N-[(3M)-3-(5-chloro-1,2,3-thiadiazol-4-yl)phenyl]-5-methyl-3-oxo-2,3-dihydro-1,2-oxazole-4-sulfonamide | C12 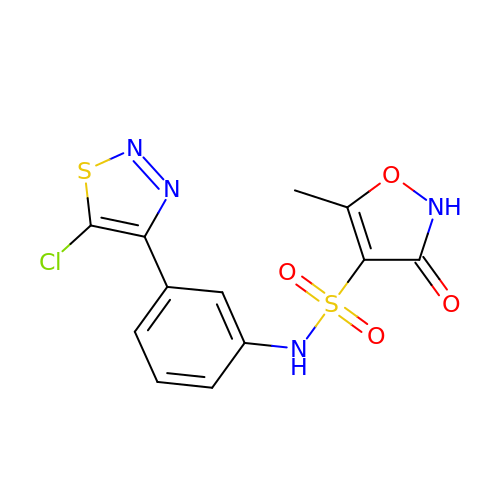H9 Cl N4 O4 S2 | DQBOCBWXJZVOII-UHFFFAOYSA-N>MRIVINGFGRIGRLVLRQILKRNSPIEVVAINDLVAGDLLTYLFKYDSTHGSFAPQATFSDGCLVMGERKVHFLAEKDVQKLPWKDLDVDVVVESTGLFVNRDDVAKHLDSGAKRVLITAPAKGDVPTFVMGVNHQ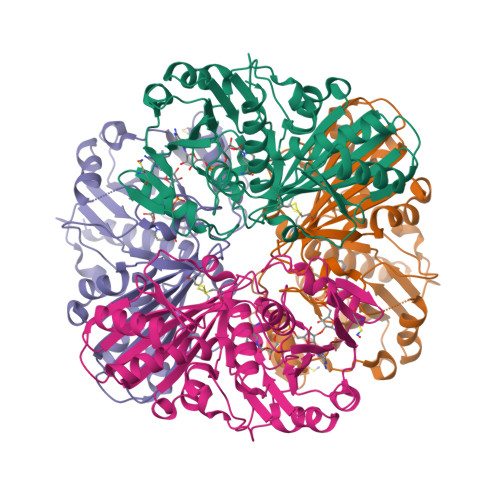QFDPADVIISNASCTTNCLAPLAKVLLDNFGIEEGLMTTVHAATATQSVVDGPSRKDWRGGRGAFQNIIPASTGAAKAVGLCLPELKGKLTGMAFRVPVADVSVVDLTVKLSSATTYEAICEAVKHAANTSMKNIMYYTEEAVVSSDFIGCEYSSVFDAQAGVALNDRFFKLVAWYDNEIGYATRIVDLLEYVQENSK[4x]(3-bromo-4-methylphenyl)boronic acid | C7 H8 B Br O2 | 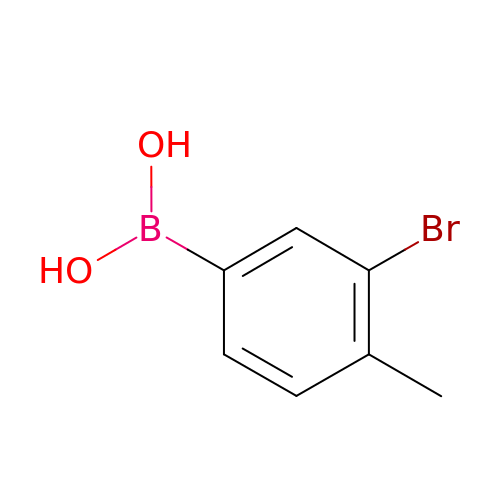VBESRPDPCSIDEN-UHFFFAOYSA-N> 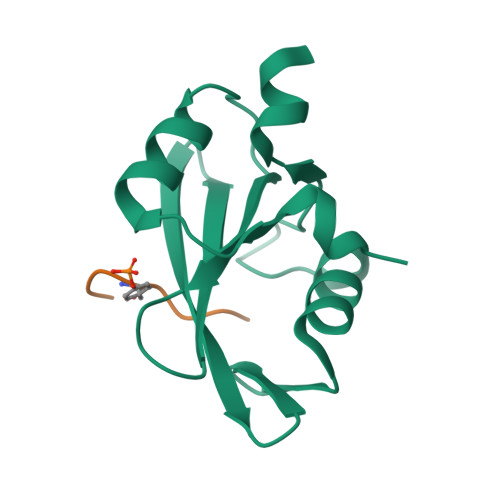SQAESKEWYHASLTRAQAEHMLMRVPRDGAFLVRKRNEPNSYAISFRAEGKIKHCRVQQEGQTVMLGNSEFDSLVDLISYYEKHPLYRKMKLRYPINEEALEKIGT;> DYGALYEGRNPGFYVEAN> MNLRI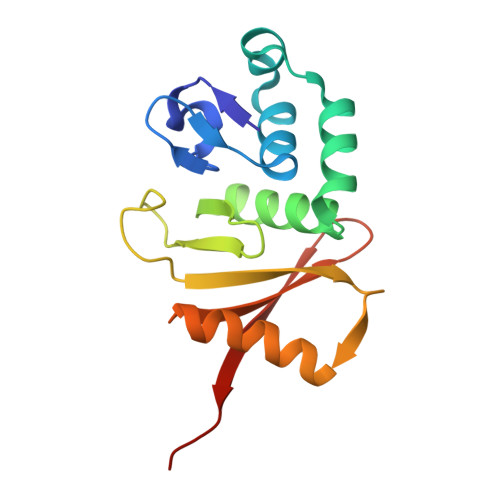PWKEVYYLGYNMGNYIKISEPELLFVLRNKPQIKDRLKLDEKTIIKEGVKKYKNFWEIYYTVKDLILRGYRVRFDGFFIELYEKGIIPGTIEQDYLVYPVSGEIRMTWGELLDIYNKAIARKSKFMLAIVDSEGDVTYYEFRKLRSNK> MGSSHHHHHHSQGSMLN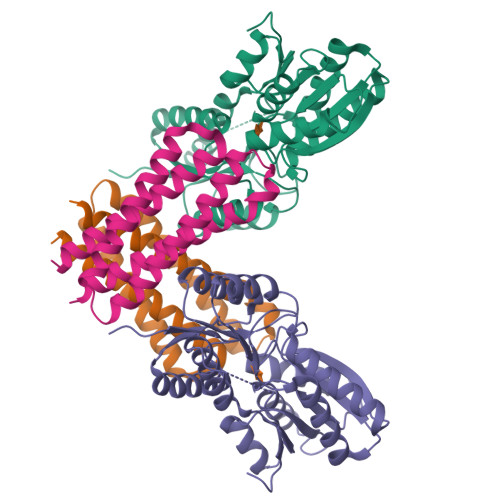NMLITNEIKQHVDSSLDNFNQYILNGTPSKKESYNNEVILAKQKIGNLKKNSDDVNQYILRDLDNTLDSYIESSKNTISAYENKEGYVFYYDDFVAAKNIASYCDAYASTLMQNFLEANSIAYKELNRNSS;> MARSNLLRDKKVEKEPIKPKIVLISHIKTNPYWLDIKAGAERAAKERGAVVEFLGPTTASTEDGLKLFDMATSAKVSGIITYVQEEGQYKKKINSAMEKGIPVVTIDSDEEDSNRIAYVGTDNVLAGQVAGKEMVKQIGTSGNVAIVMGGKNVKNQKERVEGFTQYIKSNSNLKIVDTDSSDAMLLEAEIITRKILNRNDNINALFCTSALDGIGAARAVKDLNYKDRVKIICFDDLDDTLSNIRNGLVSATIVQKSNEMGYRAVNIIMDKIEGKSNKFSKSLIDVNVINKSDVDSYKRGDDKVEN1-[7-amino-1-(pyrimidin-2-yl)indolizin-3-yl]ethanone 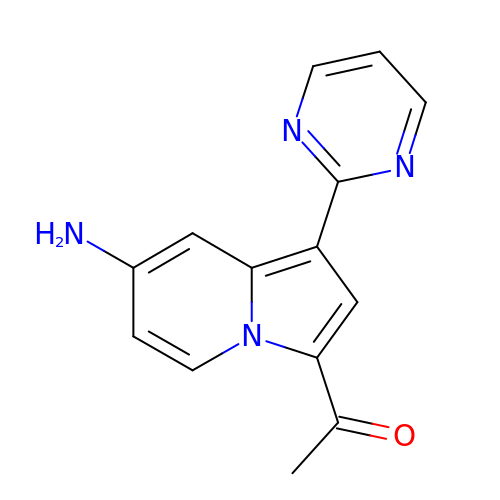| C14 H12 N4 O | PSDYTFPEBOCDIW-UHFFFAOYSA-N>[4x]GQNHHEVVKFMDVYQRSYCHPIETLVD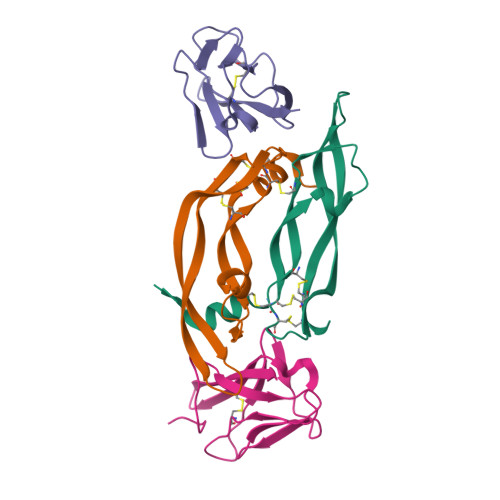IFQEYPDEIEYIFKPSCVPLMRCGGCCNDEGLECVPTEESNITMQIMRIKPHQGQHIGEMSFLQHNKCECRPKKD;>SDTGRPFVEMYSEIPEIIHMTEGRELVIPCRVTSPNITVTLKKFPLDTLIPDGKRIIWDSRKGFIISNATYKEIGLLTCEATVNGHLYKTNYLTHRQTNTI[4x]>MTPASYNLAVRRAAPAVVNVYNRGLNTNSHNQLEIRTLGSGVIMDQRGYIITNKHVINDA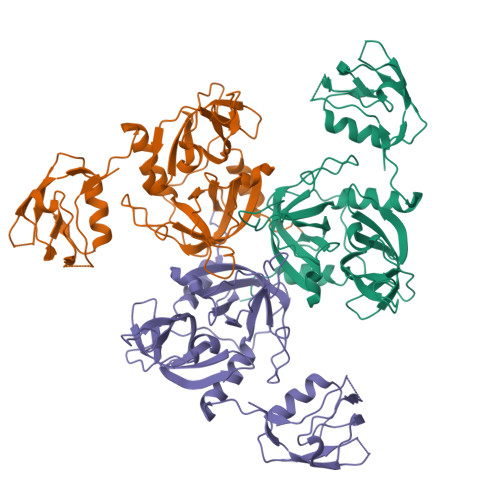DQIIVALQDGRVFEALLVGSDSLTDLAVLKINATGGLPTIPINARRVPHIGDVVLAIGNPYNLGQTITQGIISATGRIGLNPTGRQNFLQTDASINHGNSGGALVNSLGELMGINTLSFDKSNDGETPEGIGFAIPFQLATKIMDKLIRDGRVIRGYIGIGGREIAPLHAQGGGIDQLQGIVVNEVSPDGPAANAGIQVNDLIISVDNKPAISALETMDQVAEIRPGSVIPVVVMRDDKQLTLQVTIQEYPATN[3x]>MVLYFIGLGLYDERDITVKGLEIAKKCDYVFAEFYTSLMAGTTLGRIQKLI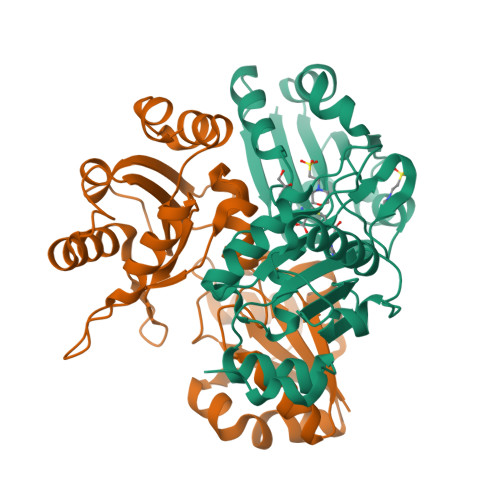GKEIRVLSREDVELNFENIVLPLAKENDVAFLTPGDPLVATTHAELRIRAKRAGVESYVIHAPSIYSAVGITGLHIYMFGKSATVAYPEGNWFPTSYYDVIKENAERGLHTLLFLDIKAEKRMYMTANEAMELLLKVEDMKKGGVFTDDTLVVVLARAGSLNPTIRAGYVKDLIREDFGDPPHILIVPGKLHIVEAEYLVEIAGAPREILRVNV[2x]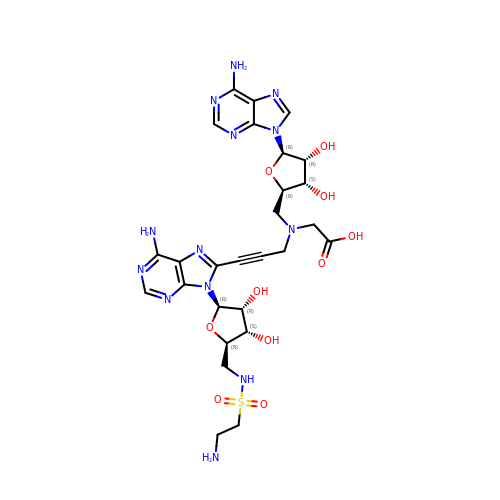2-[[(2~{R},3~{S},4~{R},5~{R})-5-(6-aminopurin-9-yl)-3,4-bis(oxidanyl)oxolan-2-yl]methyl-[3-[6-azanyl-9-[(2~{R},3~{R},4~{S},5~{R})-5-[(2-azanylethylsulfonylamino)methyl]-3,4-bis(oxidanyl)oxolan-2-yl]purin-8-yl]prop-2-ynyl]amino]ethanoic acid | C27 H35 N13 O10 S | SKWARGWQQAOVGT-GMIOVBLFSA-N>AFYLLY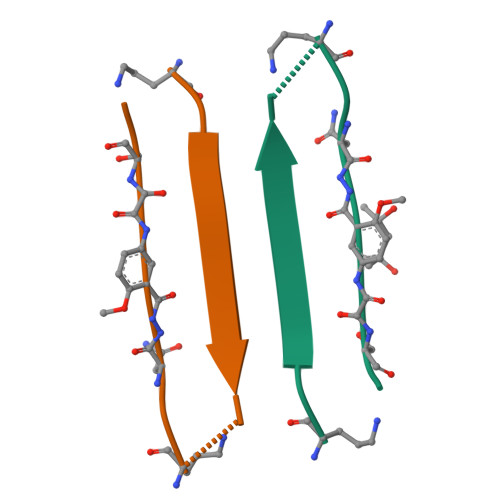YTAKNXSA[4x]(1S,5R)-7-{4-[3-(2-chloro-3,6-difluorophenoxy)propyl]phenyl}-N-cyclopropyl-N-(2,3-dichlorobenzyl)-3,9-diazabicyclo[3.3.1]non-6-ene-6-carboxamide | C33 H32 Cl3 F2 N3 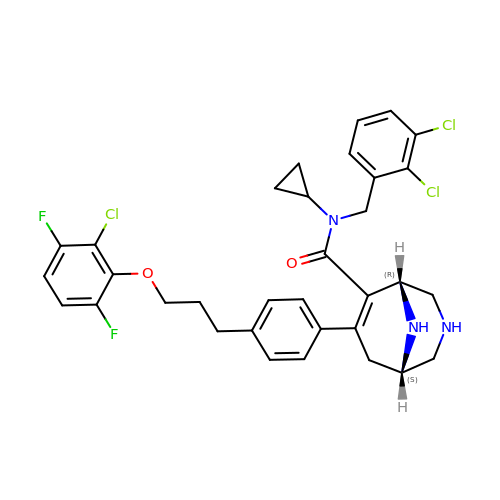O2 | SXZFQYPWEANJGQ-DWACAAAGSA-N> MAKILVVTSGKGGVGKTTTSAAIGTGLALRGFKTVIVDFDVGLRNLDLIMGCERRVVYDFVNVVNGEATLTQALIKDKRLENLHVLAASQTRDKDALTKEGVEKVMAELRKDFEYIICDSPAGIEKGAHLAMYFADEAIVVTNPEVSSVRDSDRMLGLLASKSQRAEKGEEPIKEHLLLTRYNPERVTKGEMLSVDDVEEILAIRLLGVIPESQAVLKASNQGVPVILDEQSDAGQ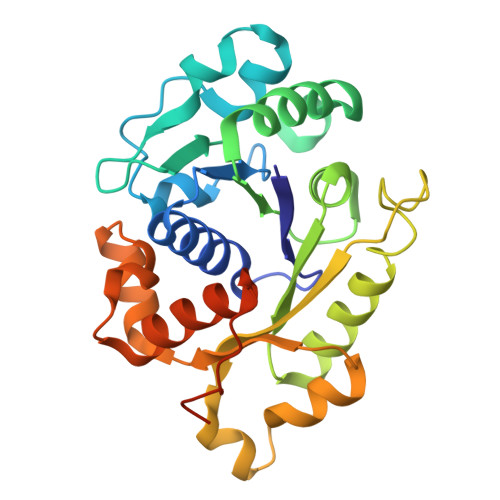AYSDAVDRLLGKEIPHRFLDVQKKGFLQRLFGGRE> GSSGSSGAAFAKILDPAYQVDKGGRVRFVVELADPKLEVKWYKNGQEIRPSTKYIFEHKGCQR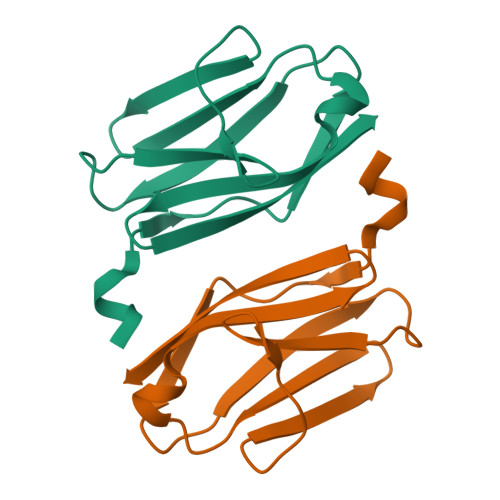ILFINNCQMTDDSEYYVTAGDEKCSTELFVRSGPSSG Cytochrome P450 enzymes (P450s) are a superfamily of monooxygenases that utilize a cysteine thiolate–ligated heme moiety to perform a wide range of demanding oxidative transformations. Within GPA biosynthesis, P450s function in a specific, stepwise manner to install the essential side-chain crosslinks in the core peptide in a process that typically requires one Oxy enzyme per crosslink to be installed. Given the apparent preference for the unusual heme orientation shown by OxyA enzymes, we investigated the OxyA homolog from kistamicin biosynthesis (OxyAkis), which is an atypical GPA. Structural and biochemical analysis of OxyAkis has shown that this P450 enzyme is highly prone to oxidation and can display an atypical heme orientation in different protein batches.

Thus, we sought to crystallize OxyAkis alone, and we were able to identify conditions in which the P450 would crystallize and diffract to high resolution (1.6 Å). With OxyAkis no longer in complex with the X-domain, we observed some changes to the flexible regions of the P450, noting that the loop connecting the F and G helices could no longer be resolved due to lack of clear density and suggesting that this loop is stabilized in the complex. Additional gaps in the structure of mobile sites surrounding the heme and active site were present, suggesting that these regions are disordered without the bound substrate, which is in keeping with results from many structurally characterized P450s. Despite these minor differences, the overall fold of OxyAkis remained largely identical to the structure previously solved in complex with the X-domain (RMSD = 0.47 Å). With the general fold essentially unchanged, we performed a detailed analysis of the active site of this P450, which revealed a mixed population of heme orientations as seen in the Fo–Fc difference map electron density at the substituent vinyl and methyl groups. Given that P450s from GPA biosynthesis are overrepresented in the structurally characterized P450s bearing the alternate heme conformation, we explored various ratios of the heme orientations that could model occupancies (2:1 ratio) of a flipped heme ligand in the structure of OxyAkis. However, even once the density of the methyl/vinyl groups was well-explained by a mixture of heme orientations; there was still evidence for additional density at the side of the heme immediately below the I-helix (β-position). Given that heme oxygenase chemistry exploits the hydroxylation of heme during its degradation, it is tempting to speculate that this density may represent hydroxylation of the heme (albeit, here the hydroxyl group would be located at a different position of the heme (β versus α position in the heme oxygenase reaction)).

> MVAPEHRVLHLRDRLDLAAELKLLCERGPLVRIPLEDGSAVHWFALGYDVVREVLGSEKFDKRVIGTHFNHQEMALPGNLLQLDPPEHTRLRRMVAPAYSVRRMQALEPRVQAIVDDHLDTMASTGPPVEFLREVAGPMAARVACEFLGIPLDDRGELIRLTAHRGGKRRRVLNGHAYLAYMRELAARLRRDPGDGMLGMVARDHGADISDEELAGLCAVVMNSSVEQTESCLAAGTLLLLEHPEQFALLRERPELGEQAVEEIVRYLSVFEGLDPRTATEDVEIGGQVIKKGEAVFCSLLAANRADPALDGFDITRKESRHVAFGHGIHHCLGAPLARMELRIAFTTLVSRFPSLRTAVPAEEIRFRPPSSNVFTLLELPLTW> MVMGIFANCIFCLKVKYLPQQQKKKLQTDIQENGGKFSFSLNPQCTHIILDNADVLSQYQLNSIQKNHVHIANPDFIWKSIREKRLLDVKNYDPYKPLDI

pmcPARP4 is an ADP-ribosyltransferase (ART) that uses NAD+ as substrate to add ADP-ribose onto target proteins, a process called mono(ADP-ribosylation) or MARylation. PARP4 is also referred to as vault PARP since it can localize to the vault particle, a cytoplasmic ribonucleoprotein complex. PARP4 has a distinct domain composition relative to other PARP enzymes; however, the N-terminal region of PARP4 is homologous to a collection of domains found in PARP1, a regulator of multiple nuclear processes including the cellular response to DNA damage. Collectively, the study establishes the human PARP4 BRCT as a nucleic acid–binding module.

We identified PARP4 lysine residues K23, K24, K31, and K36 as potentially important due to their vicinity to lysine residues important for PARP1 BRCT binding to DNA. The structures superimposed with an RMSD of 4.3 Å (comparing 74 Cα atoms) and indicated that K23 and K31 in PARP4 approximate the position of DNA polymerase μ residues that are crucial for DNA binding. We mutated lysine residues to glutamines to remove the positive charge that might interact with the negative charge on RNA/DNA, while likely maintaining the local structure by keeping a polar residue in place. We determined X-ray structures of the four PARP4 BRCT domain mutants. As expected from thermal stability analysis, the overall BRCT fold was not affected by the different mutations, and superposition of the mutant structures with WT BRCT yielded RMSD values between 0.5 and 0.8 Å (comparing all 763–788 atoms). The K31Q mutant influenced the local surface charge at the K31 position, but also influenced the placement and charge location of the K24 sidechain. The K31Q mutant showed a stronger binding deficiency with an estimated KD value of 3 ± 1 μM. The K31Q mutant showed a greater deficiency with a KD estimated at 61 ± 12 μM, and the K23/24Q mutant showed no apparent interaction. The TM of WT BRCT was measured as 51.6 °C ± 0.2 deg, whereas TM values of 54.7 °C ± 0.4 deg, 54.3 °C ± 1 deg, 58 °C ± 1 deg, and 60.0 °C ± 0.7 deg were obtained for BRCT mutants F39A, F39Q, K31Q, and K23/24Q, respectively. The mutations resulted in perturbations to electropositive regions of the BRCT surface that are expected to engage nucleic acid.Here we used a pair of thermophilic/mesophilic acylphosphatases homologues (acylphosphatase from hyperthermophilic archaeon Pyrococcus horikoshii (PhAcP) and human common-type acylphosphatase (HuAcP)) as a model to study how local flexibility of the active site affects the enzymatic activity. Despite remarkable conservation of sequence and structure at the active site, the catalytic activity of the thermophilic PhAcP is significantly poorer as compared with its mesophilic homologue HuAcP at low temperatures. The salt-bridge between the active-site residue Arg-20 and the C-terminal carboxyl group is found only in thermophilic PhAcP but not in mesophilic HuAcP. Taken together, our data suggest that the presence of the salt-bridge between the C-terminal carboxyl group and the active-site arginine residue increases the activation energy that results in a stronger temperature dependency of the enzymatic activity.

Two variants of HuAcP were constructed. Secondly, a pseudo-wild-type HuAcP (HuA99) was created by replacing the C-terminal residue with an alanine residue to resemble PhG91A. Crystal structures of HuA99 and HuG99, resolved at 1.5 Å and 1.7 Å, respectively, demonstrated that they were superimposable with a Cα r.m.s.d. value of 0.17 Å. In a good agreement with our original design, the salt-bridge between the C-terminal carboxyl group of Gly-99 and Arg-23 at the active site was only detected in HuG99, but not in the pseudo-wild-type HuA99. Regarding the Arrhenius plot, both HuG99 and HuA99 exhibited straight lines that intersected also roughly at 298 K. The salt-bridge bearing variant HuG99 illustrated a steeper slope of the Arrhenius plot, i.e. a stronger temperature dependency of the enzymatic activity, as compared to that of HuA99 lacking the salt-bridge. Importantly, the activation energy (52.5±2.5 kJmol−1) for HuG99 was analogous to that for PhWT (49.1±1.4 kJmol−1), while the activation energy for HuA99 (29.5±1.9 kJmol−1) and HuWT (37.6±3.1 kJmol−1) was comparable to that for PhG91A (32.1±1.7 kJmol−1). On the other hand, the distance was ∼6 Å throughout the simulation of PhG91A and HuA99, suggesting the salt-bridge was broken. In contrast, despite the mtm180° rotamer conformation, transitions to ptt180°, ttp180°, and mtt180° rotamers were prominent in the MD trajectories of PhG91A and HuA99. For instance, the thermophilic PhG91A is consistently less active than the mesophilic HuA99 although both enzymes lack the active-site salt-bridge. While the two enzymes have similar values of activation enthalpy (i.e. similar slope in the Arrhenius plot), the differences in enzymatic activity are a result of PhG91A having a more negative value of activation entropy.

> MAEGNTLISVDYEIFGKVQGVFFRKHTQAEGKKLGLVGWVQNTDRGTVQGQLQGPISKVRHMQEWLETRGSPKSHIDKANFNNEKVILKLDYSDFQIVA> GPSRMSADSSPLVGSTPTGYGTLTIGTSIDPLSSSVSSVRLSGYCGSPWRVIGYHVVVWMMAGIPLLLFRWKPLWGVRLRLRPCNLAHAETLVIEIRDKEDSSWQLFTVQVQTEAIGEGSLEPSPQSQAEDGRSQAAVGAVPEGAWKDTAQLHKSEEAVSVGQKRVLRYYLFQGQRYIWIETQQAFYQVSLLDHGRSCDDVHRSRHGLSLQDQMVRKAIYGPNVISIPVKSYPQLLVDEALNPYYGFQAFSIALWLADHYYWYALCIFLISSISICLSLYKTRKQSQTLRDMVKLSMRVCVCRPGGEEEWVDSSELVPGDCLVLPQEGGLMPCDAALVAGECMVNESSLTGESIPVLKTALPEGLGPYCAETHRRHTLFCGTLILQARAYVGPHVLAVVTRTGFCTAKGGLVSSILHPRPINFKFYKHSMKFVAALSVLALLGTIYSIFILYRNRVPLNEIVIRALDLVTVVVPPALPAAMTVCTLYAQSRLRRQGIFCIHPLRINLGGKLQLVCFDKTGTLTEDGLDVMGVVPLKGQAFLPLVPEPRRLPVGPLLRALATCHALSRLQDTPVGDPMDLKMVESTGWVLEEEPAADSAFGTQVLAVMRPPLWEPQLQAMEEPPVPVSVLHR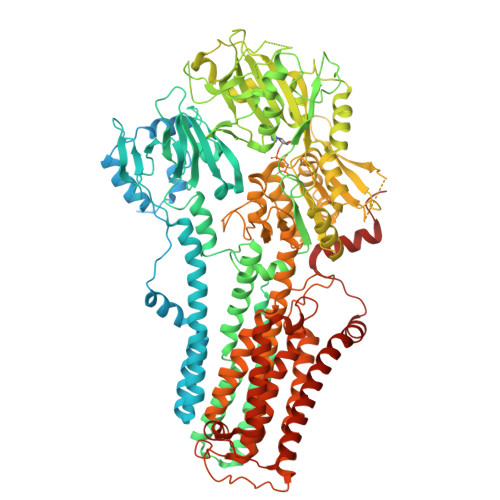FPFSSALQRMSVVVAWPGATQPEAYVKGSPELVAGLCNPETVPTDFAQMLQSYTAAGYRVVALASKPLPTVPSLEAAQQLTRDTVEGDLSLLGLLVMRNLLKPQTTPVIQALRRTRIRAVMVTGDNLQTAVTVARGCGMVAPQEHLIIVHATHPERGQPASLEFLPMESPTAVNGVKDPDQAASYTVEPDPRSRHLALSGPTFGIIVKHFPKLLPKVLVQGTVFARMAPEQKTELVCELQKLQYCVGMCGDGANDCGALKAADVGISLSQAEASVVSPFTSSMASIECVPMVIREGRCSLDTSFSVFKYMALYSLTQFISVLILYTINTNLGDLQFLAIDLVITTTVAVLMSRTGPALVLGRVRPPGALLSVPVLSSLLLQMVLVTGVQLGGYFLTLAQPWFVPLNRTVAAPDNLPNYENTVVFSLSSFQYLILAAAVSKGAPFRRPLYTNVPFLVALALLSSVLVGLVLVPGLLQGPLALRNITDTGFKLLLLGLVTLNFVGAFMLESVLDQCLPACLRRLRPKRASKKRFKQLERELAEQPWPPLPAGPLR Botulinum neurotoxins (BoNTs) are bacterial toxins produced predominantly by Clostridium botulinum. The heavy chain contains two domains: the receptor-binding domain (HC) which is responsible for targeting neuronal cells at the presynaptic neuromuscular junction, and the translocation domain (HN) which transfers the LC across the endosomal membrane within the cytosol. BoNT/B, /G, and /DC instead bind to either Synaptotagmin I or II (SytI or SytII). BoNT/B2 from Clostridium botulinum strain 111 was first identified in a case of infant botulism and initial characterization found its toxicity to be approximately 10 times lower than that of BoNT/B1.

Separate crystallization experiments containing only GD1a and HC/B2 were successful in producing crystals in the space group C121, containing the ganglioside-bound complex which diffracted to a resolution of 1.8 Å. The electron density for the entire GD1a carbohydrate is well defined. Our GD1a-bound structure of the HC domain from BoNT/B2 reveals a highly similar binding conformation of both GD1a and the HC domain when compared to BoNT/B1. Neu5Ac5 forms hydrogen bonds to N1273, N1275, G1104, N1105, G1277, and Y1263. Gal4 hydrogen bonds with His1241, I1240, S1260, and E1190, and also forms stacking interactions with W1262. GalNAc3 forms a single hydrogen bond to E1190, and Neu5Ac6 forms a single hydrogen bond to W1262. When comparing with the B1-GD1a structure, the central Gal4 superposes extremely well, but minute variations in the position of other monosaccharides are a potential result of differences in surrounding loops. One such difference is residue 1275 which is a Lys in B1 and Asn in B2. In our ganglioside-bound crystal structure, we observed a potential water-mediated interaction between N1275 and Neu5Ac5 which may result in improved binding affinity. Adjacent to N1275 is P1274 which replaces a Leu in B1 and likely provides more rigidity to the loop in an orientation that could favor interactions with the Neu5Ac5 moiety.

> SHMNSEILNNIILNLRYRDNNLIDLSGYGANVEVYDGVELNDKNQFKLTSSTNSEIRVTQNQNIIFNSMFLDFSVSFWIRIPKYKNDGIQNYIHNEYTIINCIKNNSGWKISIRGNRIIWTLTDINGKTKSVFFEYSIREDISDYINRWFFVTITNNSDNAKIYINGKLESNIDIKDIGEVIANGEIIFKLDGDIDRTQFIWMKYFSIFNTELSQSNIKEIYKIQSYSEYLKDFWGNPLMYNKEYYMFNAGNKNSYIKLKKDSSVGEILTRSKYNQNSNYINYRNLYIGEKFIIRRKSNSQSINDDIVRKEDYIYLDFFNSNREWRVYAYKDFKEEEKKLFLANIYDSNEFYKTIQIKEYDEQPTYSCQLLFKKDEESTDEIGLIGIHRFYESGIVLKDYKNYFCISKWYLKEVKRKPYNPNLGCNWQFIPKDEGWIE>MAQILPIRFQEHLQLQNLGINPANIGFSTLTMESDKFICIREKVGEQAQVVIIDMNDPSNPIRRPISADSAIMNPASKVIALKAGKTLQIFNIEMKSKMKAHTMTDDVTFWKWISLNTVALVTDNAVYHWSMEGESQPVKMFDRHSSLAGCQIINYRTDAKQKWLLLTGISAQQNRVVGAMQLYSVDRKVSQPIEGHAASFAQFKMEGNAEESTLFCFAVRGQAGGKLHIIEVGTPPTGNQPFPKKAVDVFFPPEAQNDFPVAMQISEKHDVVFL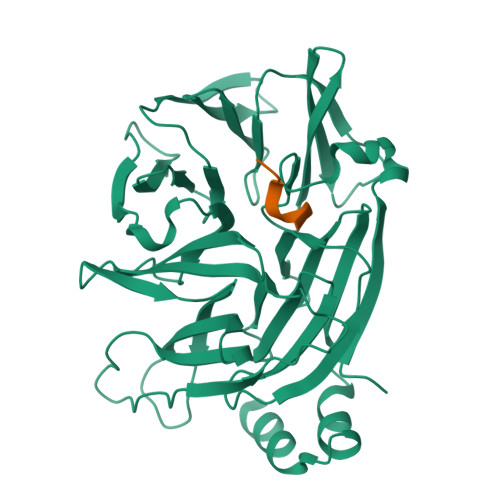ITKYGYIHLYDLETGTCIYMNRISGETIFVTAPHEATAGIIGVNRKGQVLSVCVEEENIIPYITNVLQNPDLALRMAVRNNLAGAEEL[2x];>[2x]TLPWDLWTT>MNLEKFVDELPIPEVAEPVKKNPRQTYYEIAMEEVFLKVHRDLPPTKLWTYNGSLPGPTIHANRNEKVKVKWMNKLPLKHFLPVDHTIHEGHHDEPEVKTVVHLHGGVTPASSDGYPEAWFSRDFEATGPFFEREVYEYPNHQQACTLWYHDHAMALTRLNVYAGLAGFYLISDAFEKSLELPKDEYDIPLMIMDRTFQEDGALFYPSRPNNTPEDSDLPDPSIVPFFCGETILVNGKVWPYLEVEPRKYRFRILNASNTRTYELHLDNDATILQIGSDGGFLPRPVHHQSFTIAPAERFDVIIDFSAYENKTITLKNKAGCGQEVNPETDANIMQFKVTRPLKGRAPKTLRPIFKPLPPLRPSRADQERTLTLTGTQDKYGRPILLLDNHFWNDPVTENPRLGSVEVWSIVNPTRGTHPIHLHLVQFRVIDRRPFDTEVYQSTGDIVYTGPNEAPPLHEQGYKDTIQAHAGEVIRIIARFVPYSGRYVWHCHILEHEDYDMMRPMDIIHHHHHH[2x]

Bilirubin oxidase (BOD) is another well-studied multicopper enzyme. It contains four copper ions and allows the oxidation of bilirubin as part of the heme metabolic cycle. While many redox-active enzymes are electronically isolated from their surroundings, BOD can be activated by a direct electron transfer mechanism that occurs through its T1 site. The latter acts as an internal redox mediator and by a sequential electron transfer process activates the T2/T3 site.

Here, we report the first crystal structure of the bacterial BpBOD solved at 3.5 Å resolution. The BpBOD crystal structure reveals a dimeric form. Interestingly, the BpBOD core was found to be more structured compared to the enzyme peripheral regions. As depicted, long and unstructured loops “cover” the catalytic sites, representing a large portion of the enzyme surface. Each monomer contains multi-copper T2/T3 and T1 sites having three and one copper ions, respectively. T2/T3 site residues His103, His105, His151, His153, His422, His424, His491, and His493 chelate three Cu2+ ions and exhibit high evolutionary conservation. The adjacent T1 site is comprised of residues His419, Cys492, His497, and Met502 that coordinate a single Cu2+ ion at the enzyme C’-terminal region. The revealed oxidation state of 4 Cu2+ can be correlated with the enzyme resting state. The cysteine pair Cys229 and Cys322 was found to form a disulfide bond, located 12.4 Å away from the T1 site copper ion. In total, the BpBOD sequence comprises four cysteines: one disulfide bond pair, one T1 site chelating residue (Cys492), and one oxidized Cys146 located 12 Å from the nearest T2/T3 site Cu2+ ion.>MVENKSKVKDISLAPFGKMQMEISENEMPGLMRIREEYGKDQPLKNAKITGCLHMTVECALLIETLQKLGAQIRWCSCNIYSTADYAAAAVSTLENVTVFAWKNETLEEYWWCVESALTWGDGDDNGPDMIVDDGGDATLLVHKGVEYEKLYEEKNILPDPEKAKNEEERCFLTLLKNSILKNPKKWTNIAKKIIGVSEETTTGVLRLKKMDKQNELLFTAINVNDAVTKQKYDNVYGCRHSLPDGLMRATDFLISGKIVVICGYGDVGKGCASSMKGLGARVYITEIDPICAIQAVMEGFNVVTLDEIVDKGDFFITCTGNVDVIKLEHLLKMKNNAVVGNIGHFDDEIQVNELFNYKGIHIENVKPQVDRITLPNGNKIIVLARGRLLNLGCATGHPAFVMSFSFCNQTFAQLDLWQNKDTNKYENKVYLLPKHLDEKVALYHLKKLNASLTELDDNQCQFLGVNKSGPFKSNEY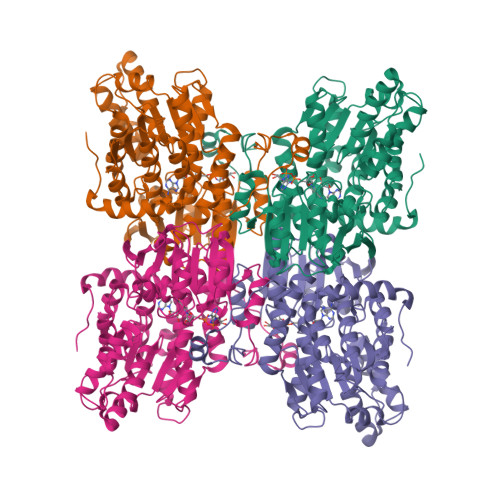RY[4x]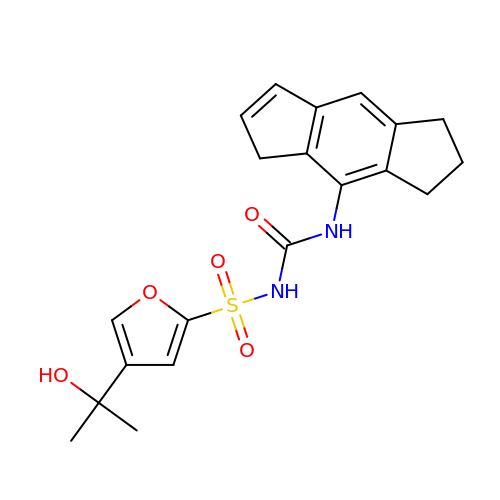1-[4-(2-oxidanylpropan-2-yl)furan-2-yl]sulfonyl-3-(1,2,3,5-tetrahydro-s-indacen-4-yl)urea | C20 H22 N2 O5 S | WBBMLFLTCGFUSC-UHFFFAOYSA-N> MGPDEPERPALLILELKSYARGVRVADAALKAAPVRLLKCKIVEPGKALIMLTGRPEDVEKAYKAALTVANKGSGNLIDSVFIPAIHPALLPFLLEETPAPPLEDPDRALLF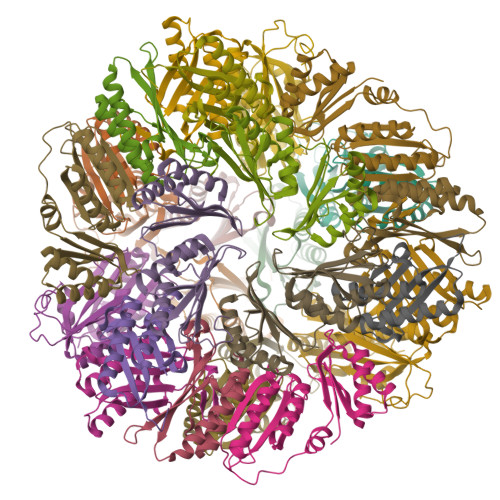VEVKTVAAAIRAADAALRAAPVELVRMRLSEHIGGKAVFALVGDPADVLRAAAVVAEVAGDQLLDIAIIPRPHPALLGREFF;> MPMLVVYVPEGYSEAQKRALLFRLAAAVVEATGTPLENVRIILTTYAPADVLLGGAIGVPLVVILVYLLEGLSPEQKAALVKALTAAAAEALGVDPENIRVILVPVPPENFGVGNGKTAAEAGGSHHWGGHHHHHH>MELFQTADWKKVKHVPVIEVLRAEGGVVEVKVSVGKEIPHPNTTEHHIAWIELVFQPEGSKFPYVVGRAEFAAHG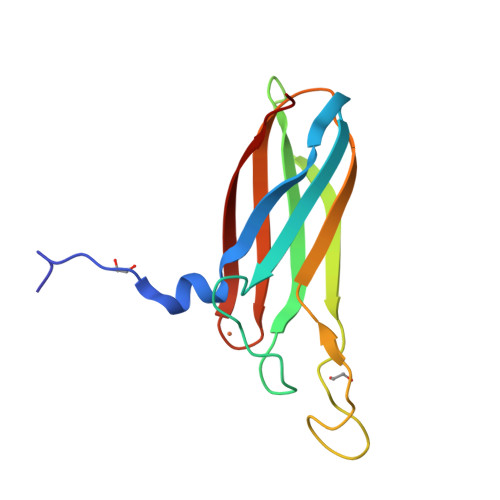ASVDGPNTSGVYTDPVAVFAFKAEKSGKLTAFSYCNIHGLWMGEATLSLE[2x]>MMPGKRRFDMLFPVDNEARQIKELNGIWKFKRDNYYKQGFEEKWFEKPLEDVIDMPVPSSYNDITTDQELRDHVGWVWYERKFAVPRLWKDQRLVLRFGSVTHHAVIYLNGKEITRHKGGFLPFEADVTEMANEGENRLTVAVGNILEWDCLPVGHIEYVRDEMHPEGQMEQKFDFDFFNYSGIHRPVRLYCTPKEYIEDISVRTTVDDKDGMVHYEIKTNAEEKFIKVYIRDEKNQVVAESNEMKDMVLVKDAQLWQPGSAYLYKLDIYFGQDHYTLPFGIRTIQLTEKQFLINGKPFYFKGFGKHEDSDIRGKGLDEALNVRDCELLKWIGANSFRTSHYPYAEEMMQMADQKGIVVIDEVPAVGMNFFDGENGGIFTEDKVNEKTLAYHKQVLKELYQRDKNHPCVVMWSITNEPHSSEEASRNYFEEVTKYIRKLDSERPITGTMNVDVEEDKISQFFDVVCINRYFGWYVGAGKIERIYPSLKTDLIKWHEKYGKPVIVTEYGADTIAGLHKLPEVIFSEEYQKRCIEENNKAMDECDFVI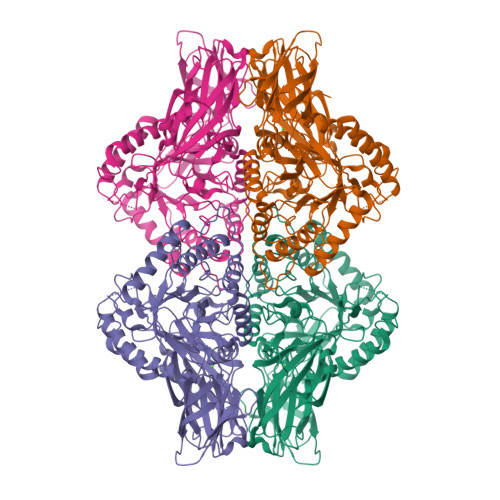GEHIWAFADFMTAFGLKRVDGNKKGIFTRERQPKTAAFAIRERWRKML[4x]> MKSLRKMLPALLILTPLLFSPAAAEEFSASFKGTDIQEFINTVSKNLNKTVIIDPSVRGTITVRSYDMLNEEQYYQFFLSVLDVYGFAVINMNNGVLKVVRAKDAKTSAVP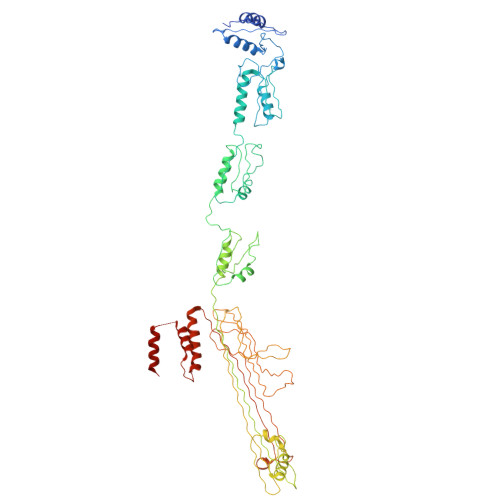VASAAAPGEGDEVVTRVVPLTNVAARDLAPLLRQLNDNAGAGSVVHYEPSNVLLMTGRAAVIKRLLTIVERVDNAGDRSVVTVPLSWASAAEVVKLVTELNKDTSKSALPGSMVANVVADERTNAVLVSGEPNSRQRIIAMIKQLDRQQAVQGNTKVIYLKYAKAADLVEVLTGISSSLQSDKQSARPVAAIDKNIIIKAHGQTNALIVTAAPDVMNDLERVIAQLDIRRPQVLVEAIIAEVQDADGLNLGIQWANKNAGMTQFTNSGLPISTAIAGANQYNKDGTISSSLASALGSFNGIAAGFYQGNWAMLLTALSSSTKNDILATPSIVTLDNMQATFNVGQEVPVLTGSQTTSGDNIFNTVERKTVGIKLKVKPQINEGDAVLLEIEQEVSSVADSASSTSSDLGATFNTRTVNNAVLVGSGETVVVGGLLDKTVTDTADKVPLLGDIPVIGALFRSDSKKVSKRNLMLFIRPTIIRDRDEYRQASSGQYTAFNNAQTKQRGKESSEASLSNDLLHIYPQQETQAFRQVSAAIDAFNLGGRP> GKDYLYDTKEENGKIISKV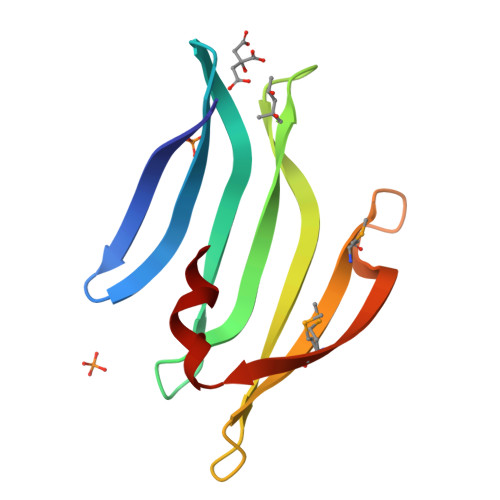VFLQENGLLNKQVRYEFQYNENGKVSEKKAFRWDRTNDEWVPFYQITYQYDDQSGEIKTNYGMWDKKKKNFSLNVQNMIIPSTNYEEIFS3'-DEOXYTHYMIDINE-5'-MONOPHOSPHATE | C10 H15 N2 O7 P | 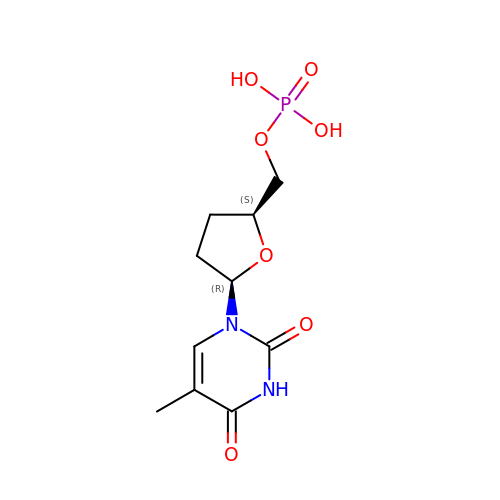WVNRRNJFRREKAR-JGVFFNPUSA-N> MIIVRYLIRETIKSQFAIFFVLFLVFLSQKFIRVLADASDGEIPTSMILSIVGLNMPAMGLLMLPLSLYIGILLTFGRLYAESEITVMNATGIGNKFLIRAALYLALITASVAAFNALWLAPW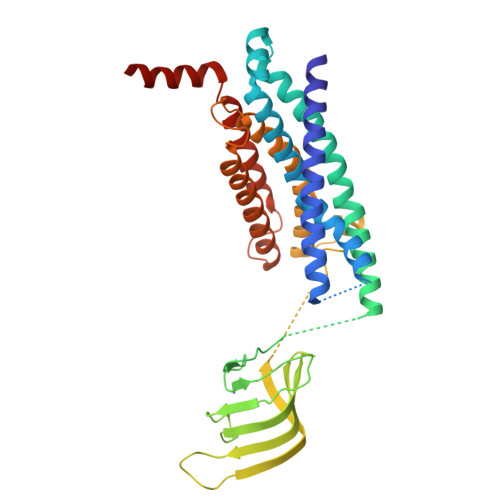SQDKEAHLMEQFAAENSVDLLQKGHFQRSPDGSSVVFIDNIENRKLYNVFVAQLAPRDSILPSVMFSHSGDVKELSDGRQIITLYDGTRYEGVPTRVDYMITNFDSYDGLIGQREVKSAERDWEALPTLSLLNNADRRAQAELQWRISLVVCIPLLTMLVVPLSAVNPRQGRFAKMGPAILIYLTYFLALSATKSAIEDGSLPVIIGLWPINAALLLAALMVNTLDSIPVRRFKDRWKQRKVA(2~{R})-2-[(4~{S})-6-(4-chlorophenyl)-8-methoxy-1-methyl-4~{H}-[1,2,4]triazolo[4,3-a][1,4]benzodiazepin-4-yl]-~{N}-ethyl-butanamide 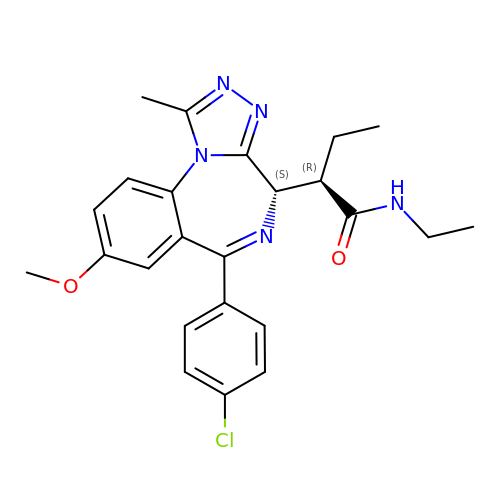| C24 H26 Cl N5 O2 | CNRGCXBSRCBICF-GCJKJVERSA-N ACETAMIDE | 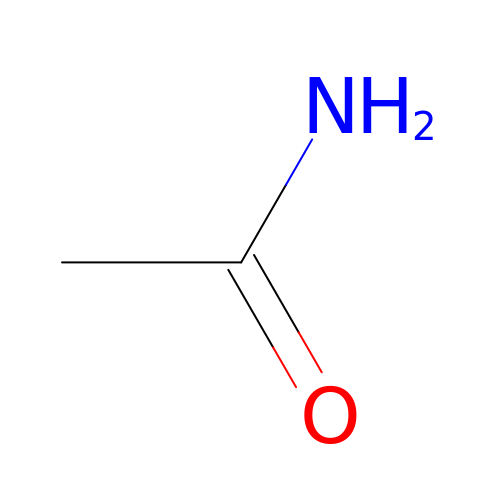C2 H5 N O | DLFVBJFMPXGRIB-UHFFFAOYSA-N> IAGGEAITTGGSRCSLGFNVSVNGVAHALTAGHCTNISASWSIGTRTGTSFPNNDYGIIRHSNPAAA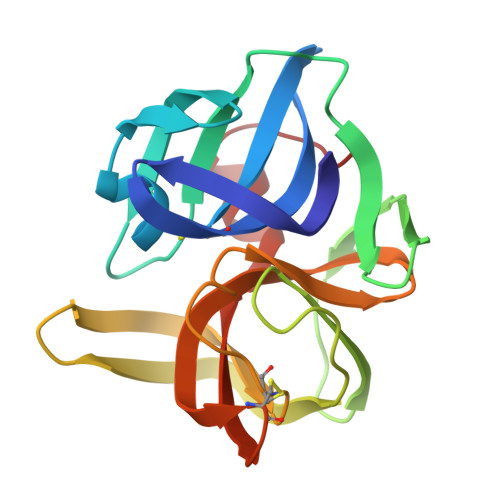DGRVYLYNGSYQDITTAGNAFVGQAVQRSGSTTGLRSGSVTGLNATVNYGSSGIVYGMIQTNVCAQPGDSGGSLFAGSTALGLTSGGSGNCRTGGTTFYQPVTEALSAYGATVL3-{(1S)-1-[(6-chloro-3,3-dimethyl-3,4-dihydroisoquinolin-1-yl)amino]-2-phenylethyl}-1,2,4-oxadiazol-5(2H)-one 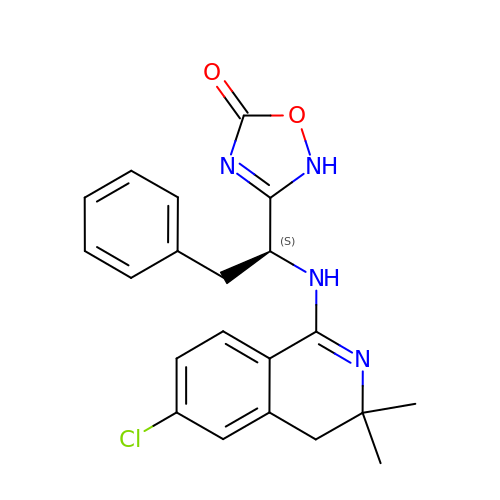| C21 H21 Cl N4 O2 | XREOSEVJCQGCHE-KRWDZBQOSA-N>TRDQNGTWEMESNENFEGWMKALDIDFALRKI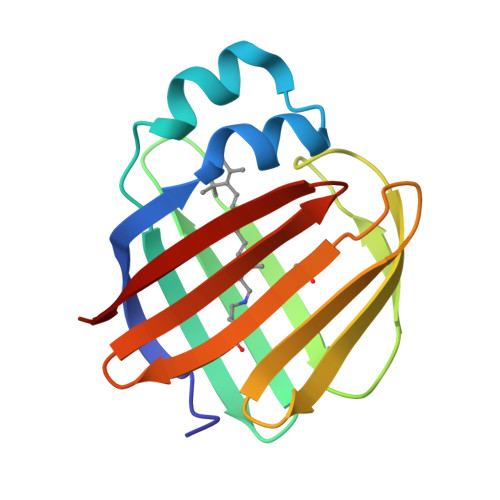AVRLTQTLVIDQDGDNFKVKCTSTFWNYDVDFTVGVEFDEYTKSLDNRHVKALVTWEGDVLVCVQKGEKENRGWKKWIEGDKLYLELTCGDQVCRQVFKKK[2x]Pyruvate carboxylase (PC) is a tetrameric enzyme that contains two active sites per subunit that catalyze two consecutive reactions. A mobile domain with an attached prosthetic biotin links both reactions, an initial biotin carboxylation and the subsequent carboxyl transfer to pyruvate substrate to produce oxaloacetate. PC is mostly found as tetramers of four identical subunits, with monomers of ~120–130 kDa in size. This enzyme possesses a tetrahedral geometry with the tetramer organized in two layers. In this work, we study the structure of Lactococcus lactis PC (LlPC) during catalysis in the presence of positive allosteric regulator acetyl-CoA.

The absence of a strong signal for the BBCP region prompted us to perform a classification with a soft mask around the BC domain of the particles aligned in the framework of the full tetramer. This unsupervised classification produced a class with 9.4% of the particles showing good signal for the BCCP domain fully engaged in the BC reaction site (BCreact) with a closed B-lid. The BC-lid is closed grabbing the MgATP where the adenine of ATP interacts with the main chain of Lys200 and Ile202, and the side chains of Glu199 and Lys157. The polyphosphate chain interacts with the amino group of Lys116, the Mg2+ ion, and residues 161-164 in the T-loop. This Mg2+ also coordinates the carboxylate groups of Glu274 and Glu286. Bicarbonate is placed between side chains of Arg290 and Glu294, and the main chain of Val293. In our cryoEM map for BCreact state biotin is placed in a catalytic position very similar to the one described previously using free biotin. The interaction between BCCP domain and the B-subdomain lid of BC is stablished only when the lid is closed through a set of point contacts, and the large tip containing the prosthetic biotin has a wide range of positions available. Noteworthy, the highest positive correlation corresponds to the BCreact pair joint by the BC-BC interaction surface, suggesting a cooperative behavior of BC regions in opposite layers to recruit biotin-carrying BCCP domains.

>[4x]VPRGSHMKKLLVANRGEIAVRVFRACNELGLSTVAVYAREDEYSVHRFKADESYLIGQGKKPIDAYLDIDDIIRVALESGADAIHPGYGLLSENLEFATKVRAAGLVFVGPELHHLDIFGDKIKAKAAADEAKVPGIPGTNGAVDIDGALEFAKTYGYPVMIKAALGGGGRGMRVARNDAEMHDGYARAKSEAIGAFGSGEIYVEKYIENPKHIEVQILGDRHGNIIHLHERDCSVQRRNQKVIEIAPAVGLSPDFRNEICEAAVKLCKNVGYVNAGTVEFLVKDDKFYFIEVNPRVQVEHTITELITGVDIVQAQILIAQGKDLHREIGLPAQSEIPLLGSAIQCRITTEDPQNGFLPDTGKIDTYRSPGGFGIRLDVGNAYAGYEVTPYFDSLLVKVCTFANEFSDSVRKMDRVLHEFRIRGVKTNIPFLINVIANENFTSGQATTTFIDNTPSLFNFPRLRDRGTKTLHYLSMITVNGFPGIENTEKRHFEEPRQPLLNLEKKKTAKNILDEQGADAVVDYVKNTKEVLLTDTTLRDAHQSLLATRLRLQDMKGIAQAIDQGLPELFSAEMWGGATFDVAYRFLNESPWYRLRKLRKLMPNTMFQMLFRGSNAVGYQNYPDNVIEEFIRVAAHEGIDVFRIFDSLNWLPQMEKSIQAVRDNGKIAEATICYTGDILDPSRPKYNIQYYKDLAKELEATGAHILAVKDMAGLLKPQAAYRLISELKDTVDLPIHLHTHDTSGNGIITYSGATQAGVDIIDVATASLAGGTSQPSMQSIYYALEHGPRHASINVKNAEQIDHYWEDVRKYYAPFEAGITSPQTEVYMHEMPGGQYTNLKSQAAAVGLGHRFDEIKQMYRKVNMMFGDIIKVTPSSKVVGDMALFMIQNDLTEEDVYARGNELNFPESVVSFFRGDLGQPVGGFPEKLQKIIVKDKAVITDRPGLHAEKVDFETVKADLEQKIGYEPGDHEVISYIMYPQVFLDYQKMQREFGAVTLLDTPTFLHGMRLNEKIEVQIEKGKTLSIRLDEIGEPDLAGNRVLFFNLNGQRREVVINDQSVQAQVVAKRKAETGNPNQIGATMPGSVLEILVKAGDKVQKGQALMVTEAMKMETTIEAPFDGEIVDLHVVKGEAIQTQDLLIEIN>[2x]QSACTLQSETHPPLTW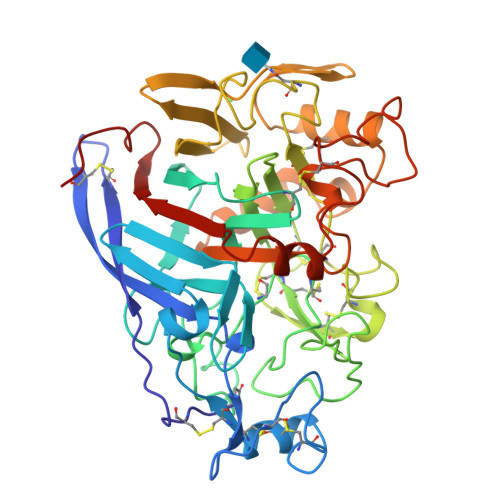QKCSSGGTCTQQTGSVVIDANWRWTHATNSSTNCYDGNTWSSTLCPDNETCAKNCCLDGAAYASTYGVTTSGNSLSIDFVTQSAQKNVGARLYLMASDTTYQEFTLLGNEFSFDVDVSQLPCGLNGALYFVSMDADGGVSKYPTNTAGAKYGTGYCDSQCPRDLKFINGQANVEGWEPSSNNANTGIGGHGSCCSEMNIWEANSISEALTPHPCTTVGQEICEGDGCGGTYSDNRYGGTCDPDGCDWNPYRLGNTSFYGPGSSFTLDTTKKLTVVTQFETSGAINRYYVQNGVTFQQPNAELGSYSGNELNDDYCTAEEAEFGGSSFSDKGGLTQFKKATSGGMVLVMSLWDDYYANMLWLDSTYPTNETSSTPGAVRGSCSTSSGVPAQVESQSPNAKVTFSNIKFGPIGSTGNPSG> GSHMTNVRAHAQANQAASNLQDDWANGKRSPGSFEPGQGFALLHIPKLDVVVPIAEGISSKKVLDRGMVGHYAEDGLKTAMPDAKAGNFGLAGHRNTHGEPFRYINKLEPGDPIVVETQDKYFVYKMASILPVTSPSNVSVLDPV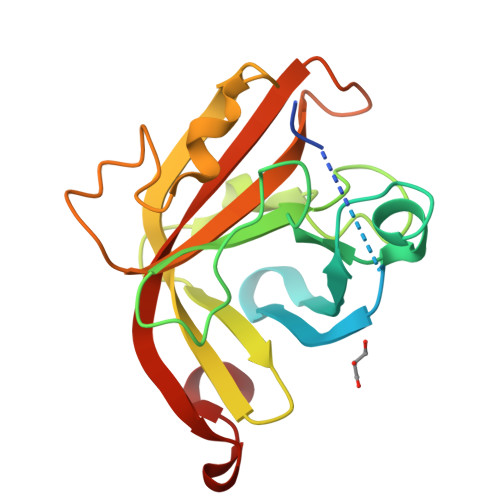PKQSGFKGPGRYITLTTCTPEFTSKYRMIVWGKMVEERPRSKGKPDALVS> SANTNHQYAVIAYFYGNASLQGANATINIWEPNLKNPNGDFSLTQIWISAGSGSSLNTIEAGWQVYPGRTGDSQPRFFIYWTADGYTSTGCYDLTCPGFVQTNNYYAIGMALQPSVYGGQQYELNESIQRDPATGNWWLYLWGTVVGYWPASIYNSITNGADTVEWGGEIYDSSGTGGFHTTTQMGSGHFPTEGYGKASYVRDLQCVDTYGNVISPTANSFQGIAPAPNCYNYQFQQGSSELYLFYGGPGCQAIAHHHHHH;> GGGG

Neprosin from the pitcher plant is a reported prolyl endopeptidase. Here, we produce recombinant neprosin and its mutants, and find that full-length neprosin is a zymogen, which is self-activated at gastric pH by the release of an all-β pro-domain via a pH-switch mechanism featuring a lysine plug. The catalytic domain is an atypical 7+8-stranded β-sandwich with an extended active-site cleft containing an unprecedented pair of catalytic glutamates. Neprosin efficiently degrades both gliadin and the 33-mer in vitro under gastric conditions and is reversibly inactivated at pH > 5.

The final refined model of the derivative complex was used to solve the native pro-neprosin structure by molecular replacement. Moreover, mature neprosin produced two different monoclinic crystal forms, I and II, whose structures were likewise solved by molecular replacement. Crystal form II, in turn, was practically indistinguishable from crystal form I (core RMSD = 0.66 Å) except for the tip of loop Lβ21β22, which was spaced apart by 3.8 Å, and the C-terminal tag, which was reoriented owing to crystal packing. Moreover, in the structures of mature neprosin crystal forms I and II, the C-terminal segment, which spanned an alanine–isoleucine–alanine tripeptide followed by the His6-tag, ran along the surface of a symmetry mate, thus mimicking a product complex. Both crystal forms were monoclinic but with different cell constants, which resulted in variable crystal packing. Even so, the C-terminal tag penetrates the cleft in a similar manner in both crystallographic arrangements but is shifted by three positions, so that H404–H409 from crystal form I overlaps A401–H406 from crystal form II. Indeed, we found a striking pair of glutamate residues (E188 and E297) bridged by a solvent molecule pinching the bound peptides in the product complexes. In crystal form II, a clearly resolved second solvent molecule would replace the scissile carbonyl oxygen of a substrate. Our results suggest that the mature neprosin structures mimic upstream product complexes collectively occupying subsites S6 to S1′, with the two catalytic glutamates plus the bridging solvent molecule poised for reaction.>[2x]GSLNITENESISTAVIDAINSGATLKDINAIPDDMMDDIYSYAYDFYNKGRIEEAEVFFRFLCIYDFYNVDYIMGLAAIYQIKEQFQQAAD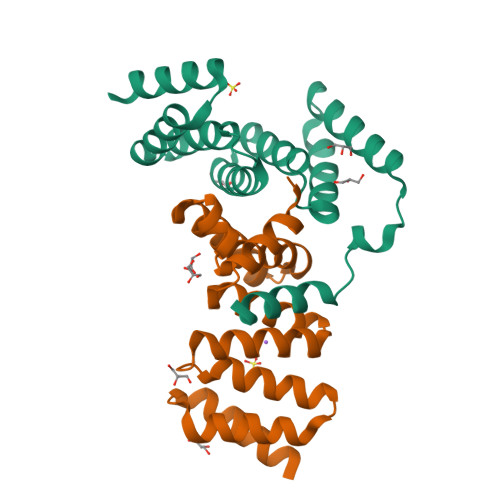LYAVAFALGKNDYTPVFHTGQCQLRLKAPLKAKECFELVIQHSNDEKLKIKAQSYLDAIQ>ANPLYQKHIISINDLSRDDLNLVLATAAKLKANPQPELLKHKVIASCFFEASTRTRLSFETSMHRLGASVVGFSDSANTSLGKKGETLADTISVISTYVDAIVMRHPQEGAARLATEFSGNVPVLNAGDGSNQHPTQTLLDLFTIQETQGRLDNLHVAMVGDLKYGRTVHSLTQALAKFDGNRFYFIAPDALAMPQYILDMLDEKGIAWSLHSSIEEVMAEVDILYMTRVQKERLDPSEYANVKAQFVLRASDLHNAKANMKVLHPLPRVDEIATDVDKTPHAWYFQQAGNGIFARQALLALVLNRDLVL[2x];>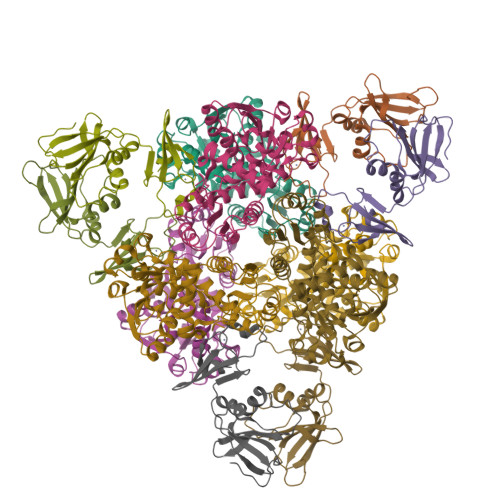MTHDNKLQVEAIKRGTVIDAIPAQIGFKLLSLFKLTETDQRITIGLNLPSGEMGRKDLIKIENTFLSEDQVDQLALYAPQATVNRIDNYEVVGKSRPSLPERIDNVLVCPNSNCISHAEPVSSSFAVRKRANDIALKCKYCEKEFSHNVVLAN[2x]> VGSLNCIVAVSQNMGIGKNGDLPWPPLRNEFRYFSRMTTTSSVEGKQNLVIMGKKTWFSIPEKSRPLKGRINLVLSRELKEPPQGAH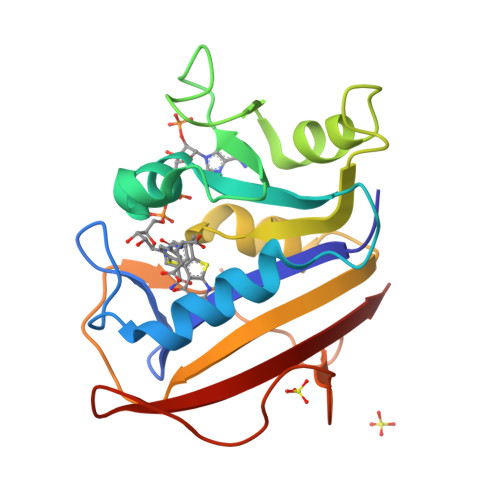FLSRSLDDALKLTEQPELANKVDMVWIVGGSSVYKEAMNHPGHLKLFVTRIMQDFESDTFFPEIDLEKYKLLPEYPGVLSDVQEEKGIKYKFEVYEKND>[3x]MHHHHHHGMLKGGVIMDVVTPEQAKIAEKSGACAVMALESIPADMRKSGKVCRMSDPKMIKDIMNSVSIPVMAKVRIGHFVEAQIIEALEVDYIDESEVLTPADWTHHIEKDKFKVPFVCGAKDLGEALRRINEGAAMIRTKGEAGTGDVSEAVKHIRRITEEIKACQQLKSEDDIAKVAEEM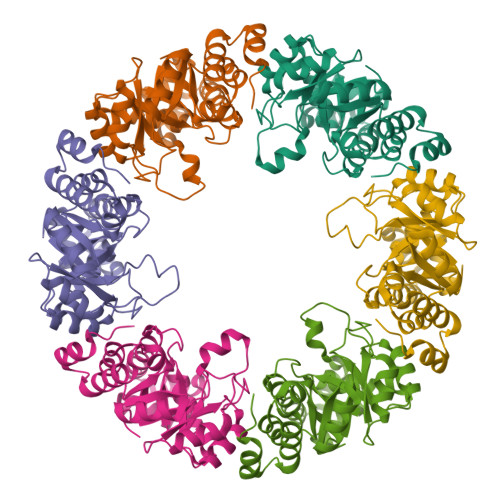RVPVSLLKDVLEKGKLPVVNFAAGGVATPADAALLMQLGCDGVFVGSGIFKSSNPVRLATAVVEATTHFDNPSKLLEVSSDLGELMGGVSIESISHASNGVRLSEIGW> MDSQRNLLVIALLFVSFMIWQAWEQDKNPQPQAQQTTQTTTTAAGSAADQGVPASGQGKLISVKTDVLDLTINTRGGDVEQALLPAYPKELNSTQPFQLLETSPQFIYQAQSGLTGRDGPDNPANGPRPLYNVEKDAYVLAEGQNELQVPMTYTDAAGNTFTKTFVLKRGDYAVNVNYNVQNAGEKPLEISSFGQLKQSITLPPHLDTGSSNFALHTFRGAAYSTPDEKYEKYKFDTIADNENLNISSKGGWVAMLQQYFATAWIPHNDGTNNFYTANLGNGIAAIGYKSQPVLVQPGQTGAMNSTLWVGPEIQDKMAAVAPHLDLTVDYGWLWFISQPLFKLLKWIHSFVGNWGFSIIIITFIVRGIMYPLTKAQYTSMAKMRMLQPKIQAMRERLGDDKQRISQEMMALYKAEKVNPLGGCFPLLIQMPIFLALYYMLMGSVELRQAPFALWIHDLSAQDPYYILPILMGVTMFFIQKMSPTTVTDPMQQKIMTFMPVIFTVFFLWFPSGLVLYYIVSNLVTIIQQQLIYRGLEKRGLHSREKKKS;> MENLNMDLLYMAAAVMMGLA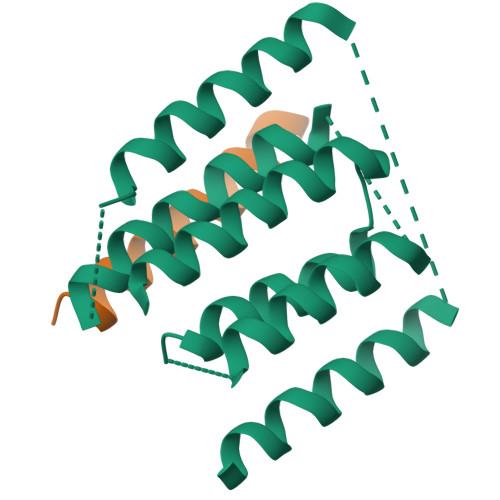AIGAAIGIGILGGKFLEGAARQPDLIPLLRTQFFIVMGLVDAIPMIAVGLGLYVMFAVA>[2x]LEIWELKKDVYVVELDWYPDAPGEMVVLTCDTPEEDGITWTLDQSSEVLGSGKTLTIQVKEFGDAGQYTCHKGGEVLSHSLLLLHKKEDGIWSTDILKDQKEPKNKTFLRCEAKNYSGRFTCWWLTTI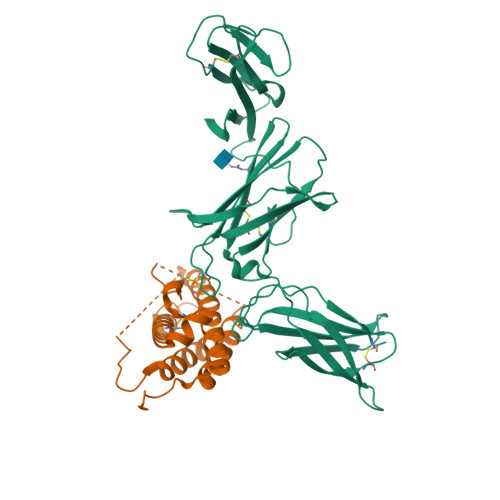STDLTFSVKSSRGSSDPQGVTCGAATLSAERVRGDNKEYEYSVECQEDSACPAAEESLPIEVMVDAVHKLKYENYTSSFFIRDIIKPDPPKNLQLKPLKNSRQVEVSWEYPDTWSTPHSYFSLTFCVQVQGKSKREKKDRVFTDKTSATVICRKNASISVRAQDRYYSSSWSEWASVPCSHHHHHH;>LRAVPGGSSPAWTQCQQLSQKLCTLAWSAHPLVGHMDLREEGDEETTNDVPHIQCGDGCDPQGLRDNSQFCLQRIHQGLIFYEKLLGSDIFTGEPSLLPDSPVGQLHASLLGLSQLLQPEGHHWETQQIPSLSPSQPWQRLLLRFKILRSLQAFVAVAARVFAHGAATLSPHHHHHH[2x]> ANIVGGIEYSINNASLCSVGFSVTRGATKGFVTAGHCGTVNATARIGGAVVGTFAARVFPGNDRAWVSLTSAQTLLPRVANGSSFVTVRGSTEAAVGAAVCRSGRTTGYQCGTITAKNVTANYAEGAVRGLTQGNACMGRGD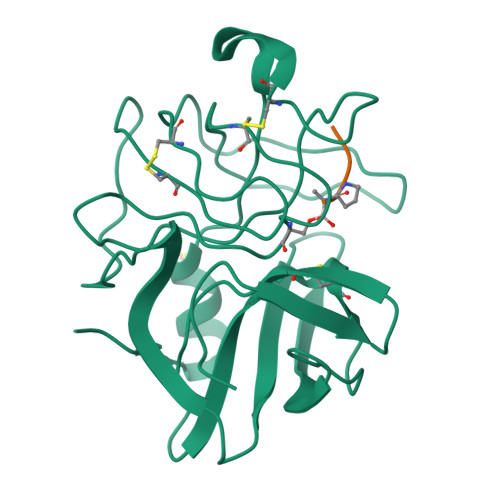SGGSWITSAGQAQGVASGGNVQSNGNNCGIPASQRSSLFERLQPILSQYGLSLVTG;> XAAPA>MSLTTPTMIAAVVEEANGPFVLRKLARPQPAPGQVLVQIEASGTNPLDAKIRAGEAPHAQQPLPAILGMDLAGTVVAVGPEVDSFRVGDAVFGLTGGV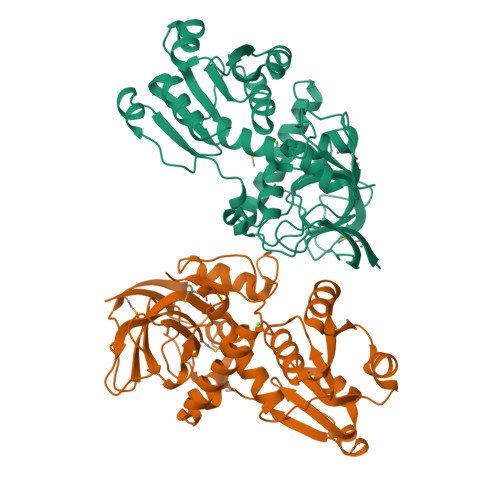GGLQGTHAQFAAVDARLLASKPAALTMRQASVLPLVFITAWEGLVDRAQVQDGQTVLIQGGGGGVGHVAIQIALARGARVFATARGSDLEYVRDLGATPIDASREPEDYAAEHTAGQGFDLVYDTLGGPVLDASFSAVKRFGHVVSCLGWGTHKLAPLSFKQATYSGVFTLHTLLANEGLAHFGEMLREADALVQTGKLAPRLDPRTFSIAEIGSAYDAVLGRNDVPRQRGKIAITVEGHHHHHH[2x]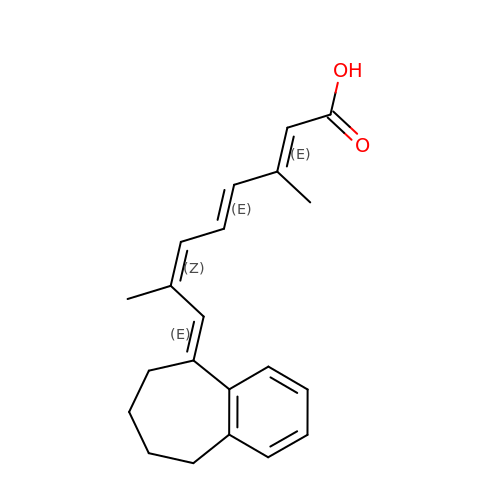(2E,4E,6Z,8E)-3,7-dimethyl-8-(6,7,8,9-tetrahydro-5H-benzo[7]annulen-5-ylidene)octa-2,4,6-trienoic acid | C21 H24 O2 | GVIXTTYIECEGAU-IVVJPBLYSA-N>GMSVIKPDMKIKLRMEGAVNGHPFAIEGVGLGKPFEGKQSMDLKVKEGGPLPFAYDILTMAFCYGNRVFAKYPENIVDYFKQSFPEGYSWERSMIYEDGGICNATNDITLDGDCYICEIRFDGVNFPANGPVMQKRTVKWELSTEKLYVRDGVLKSDGNYALSLEGGGHYRCDFKTTYKAKKVV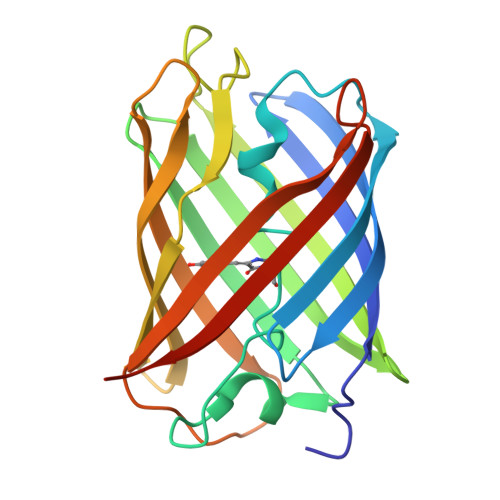QLPDYHSVDHHIEIISHDKDYSNVNLHEHAEAHSELPRQAK[8x]methyl 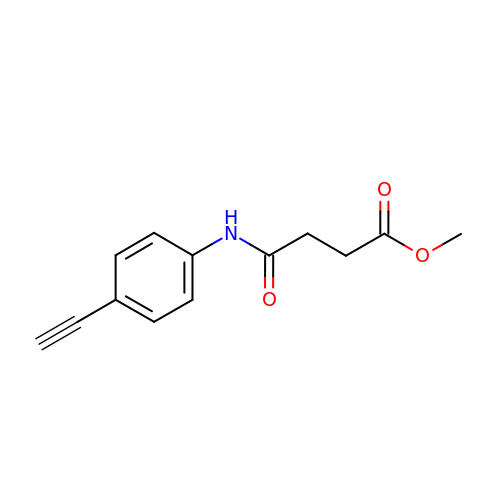4-[(4-ethynylphenyl)amino]-4-oxidanylidene-butanoate | C13 H13 N O3 | HMVIXCAGQZCUNY-UHFFFAOYSA-N> VLCAYVEDPTKSDPPSSSTDQPTTTFTAIDRWYTGRLNSWTKAVKTFSFQAVPLPGAFLSRQGGLNGGAFTATLHRHFLMKCGWQVQVQCNLTQFHQGALLVAMVPETTLDVKPDGKAKSLQELNEEQWVEMSDDYRTGKNMPFQSLGTYYRPPNWTWGPNFINPYQVTV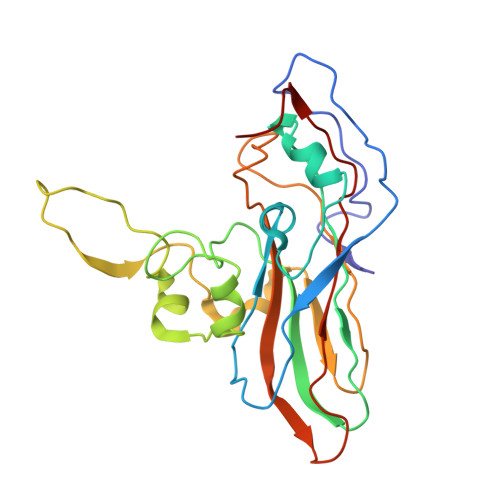FPHQILNARTSTSVDINVPYIGETPTQSSETQNSWTLLVMVLVPLDYKEGATTDPEITFSVRPTSPYFNGLRNRYT> MTGNPDPNANPNVDPNANPNANPNANPNANPNANPNAEPSDKHIKEYLNKIQNSLSTEWSPCSVTCGNGIQVRIKPGSANKPKDELDYANDIEKKICKMEKCSSVFNVVNSGGSGTENHKDDAVLLKHGWCEMLKGGVIMDVKSVEQAKIAEEAGAIGVMVLENIPSELRNKEGVARSVDPSKVEEIKKCVSINVLARVRIGH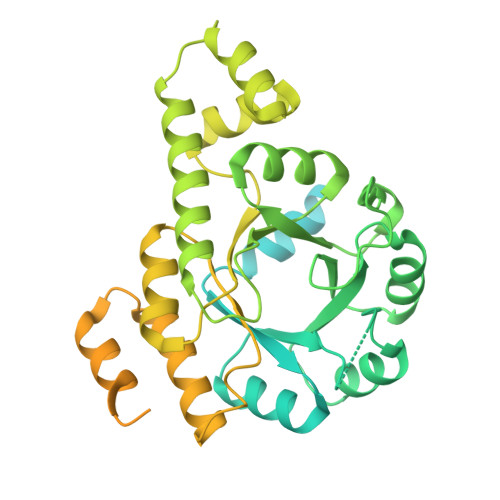FVEAQILEELKIDMIDESEVLTIADEMHHIDKHKFKTPFVCGCTNLGEALRRISEGASMIRTKGEAGTGNIIEAIKHIRTVNNEICYLCCLSDSEVYHFAKKINAPIDLVLLTKKLKRLPVVNFAAGGVATPADAAMCMQLGMDGVFVGSGIFESENPRKMAASIVSAVSNFNNPKILLDVSMNLGKAMCGSTRVSDKWKNKNEEHTKFLTPQTGNPDPNANPNVDPNANPNANPNANPNANPNANPNAEPSDKHIKEYLNKIQNSLSTEWSPCSVTCGNGIQVRIKPGSANKPKDELDYANDIEKKICKMEKCSSVFNVVNSGGSLEHHHHHH>[2x]MARTFFVGGNFKLNGSKQSIKEIVER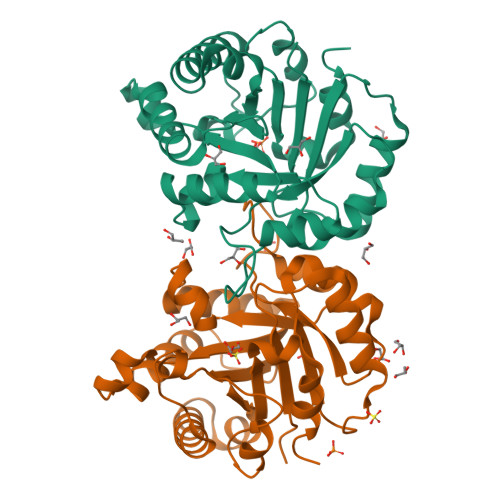LNTASIPENVEVVICPPATYLDYSVSLVKKPQVTVGAQNAYLKASGAFTGENSVDQIKDVGAKWVILGHSERRSYFHEDDKFIADKTKFALGQGVGVILSIGETLEEKKAGKTLDVVERQLNAVLEEVKDWTNVVVAYEPVWAIGTGLAATPEDAQDIHASIRKFLASKLGDKAASELRILYGGSANGSNAVTFKDKADVDGFLVGGASLKPEFVDIINSRN>MVQEIDLGLTCDMHVHVREGAMCELVTPKIRDGGVSIAYIMPNLQPPITTLDRVIEYKKTLQKLAPKTTFLMSFYLSKDLTPDLIHEAAQQHAIRGVKCYPAGVTTNSAAGVDPNDFSAFYPIFKAMQEENLVLNLHGEKPSVHDGDKEPIHVLNAEEAFLPALKKLHNDFPNLKIILEHCTSESAIKTIEDINKNVKKATDVKVAATLTAHHLFLTIDDWAGNPVNFCKPVAKLPNDKKALVKAAVSGKPYFFFGSDSAPHPVQNKANYEGVCAGVYSQSFAIPYIAQVFEEQNALENLKGF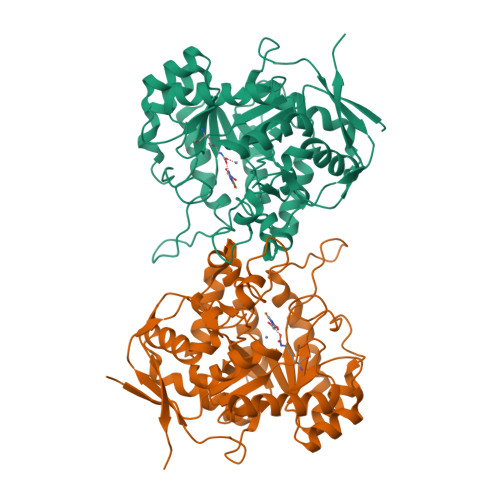VSDFGISFYEVKDSEVASSDKAILFKKEQVIPQVISDGKDISIIPFKAGDKLSWSVRWEPRLEHHHHHH[4x]>[6x]MRDWKTN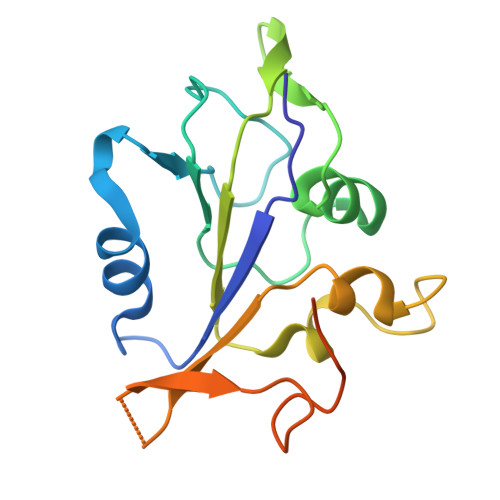VHVIVGPPGCGKSKWAANFADPETTYWKPPRNKWWDGYHGEEVVVIDDFYGWLPWDDLLRLCDRYPLTVETKGGTVPFLARSILITSNQTPLEWYSSTAVPAVEALYRRITSLVFWKNATEQSTEEGGQFVTLSPPCPEFPYEINYGSLEHHHHHH>[2x]MEVCNDEVDLYLLMDCSGSIRRHNWVKHAVPLAMKLIQQLNLNENAIHLYANIFSNNAKEIIRLHSDASKNKEKALIIIKSLLSTNLPYGRTNLSDALLQVRKHLNDRINRENANQ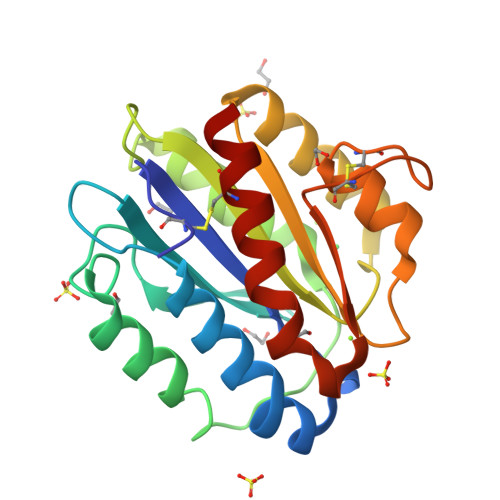LVVILTDGIPDSIQDSLKESRKLNDRGVKIAVFGIGQGINVAFNRFLVGCHPSDGKCNLYADSAWENVKNVIGPFMKAVCVEVEKTA>MSSGKKPVKVKTPAGKEAELVPEKVWALAPKGRKGVKIGL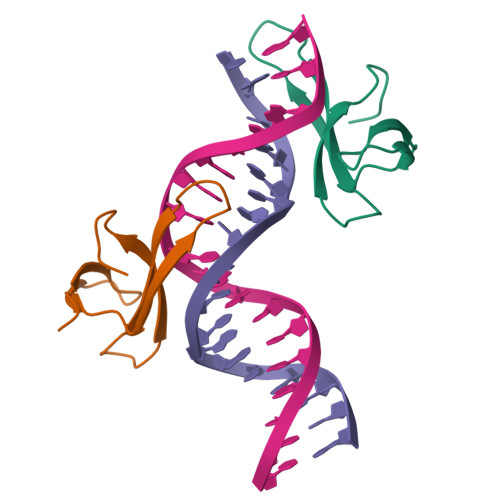FKDPETGKYFRHKLPDDYPI[2x]> SMNPPAGPVRAIAEYERSAAVLVRYPFGIPMELIKELAKNDKVITIVASESQKNTVITQYTQSGVNLSNCDFIIAKTDSYWTRDYTGWFAMYDTNKVGLVDFIYNRPRPNDDEFPKYEAQYLGIEM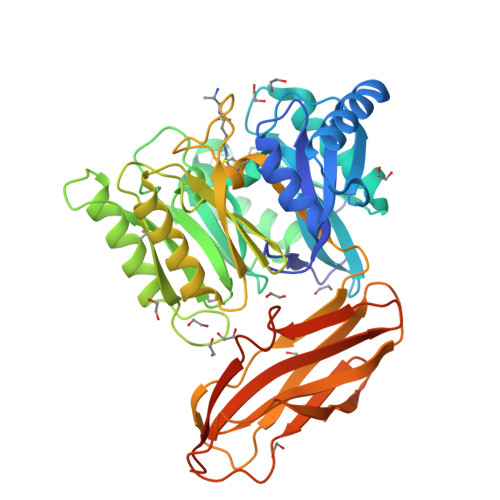FGMKLKQTGGNYMTDGYGSAVQSHIAYTENSSLSQAQVNQKMKDYLGITHHDVVQDPNGEYINHVDCWGKYLAPNKILIRKVPDNHPQHQALEDMAAYFAAQTCAWGTKYEVYRALATNEQPYTNSLILNNRVFVPVNGPASVDNDALNVYKTAMPGYEIIGVKGASGTPWLGTDALHCRTHEVADKGYLYIKHYPILGEQAGPDYKIEADVVSCANATISPVQCYYRINGSGSFKAADMTMESTGHYTYSFTGLNKNDKVEYYISAADNSGRKETYPFIGEPDPFKFTCMNETNTCTVTGAAKALRAWFNA>[2x]MQFPQLDPATLAAFSAAFRGELIWPSDADYDEARRIWNGTIDRRPALIARCTSTPDVVAAVSFARKSGLLVAVRGGGHSMAGHSVCDGGIVIDLSLMNSIKVSRRLRRARAQGGCLLGAFDTATQAHMLATPAGVVSHTGLGGMVLGGGFGWLSRKYGLSIDNLTSVEIVTADGGVLTASDTE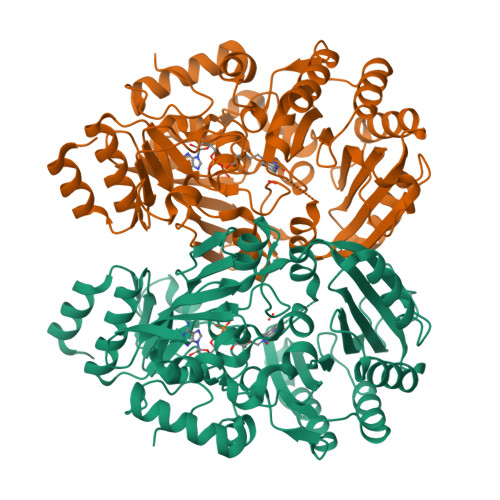NPDLFWAVRGGGGNFGVVTAFEFDLHRVGPVRFASTYYSLDEGPQVIRAWRDHMATAPDELTWALYLRLAPPLPELPADMHGKPVICAMSCWIGDPHEGERQLESILHAGKPHGLTKATLPYRALQAYSFPGAVVPDRIYTKSGYLNELSDEATDTVLEHAADIASPFTQLELLYLGGAVARVPDDATAYPNRQSPFVTNLAAAWMDPTEDARHTAWAREGYRALAGHLSGGYVNFMNPGEADRTREAYGAAKFERLQGVKAKYDPTNLFRLNQNIPPSSP> MSTPDAVDKYLETPGDENEHAHFQKAKERLEAKHRERM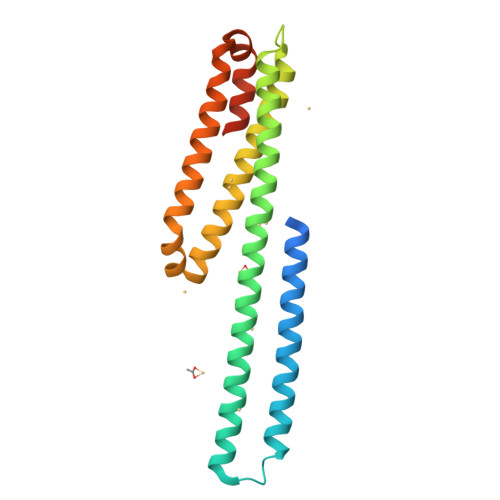SQVMREWEEAERQAKNLPKADKKAVIQHFQEKVESLEQEAANERQQLVETHMARVEAMLNDRRRLALENYITALQAVPPRPRHVFNMLKKYVRAEQKDRQHTLKHFEHVRMVDPKKAAQIRSQVMTHLRVIYERMNQSLSLLYNVPAVAEEIQDEVDELLQKEQNYSDDIEGR Progenitor sequence of the assigned 28 sequences was generated by ancestral sequence reconstruction, and the generated sequence exhibited L-lysine oxidase activity; thus, we named the enzyme AncLLysO. AncLLysO has a fold typical of the flavin-dependent amine oxidase (FAO) superfamily —the Rossmann-core fold, which recognizes FAD, and a hot-dog-like fold, which is important for the recognition of substrates. Taken together, we assigned a novel FAD-dependent enzyme, called LLysO and bearing a main L-Lys α-oxidase and promiscuous monooxygenase activity, from the database. The main-chain amino group of L-Lys is deprotonated by an activated solvent water molecule, and the hydride on the main-chain carbon atom is transferred to FAD.

In this study, the crystal structure for the ligand-free form of AncLLysO (AncLLysO(LF)) was determined at a 2.4-Å resolution. The initial phase was determined using the iodide single anomalous dispersion (SAD) method. The active site structure of AncLLysO(LF) indicated that residues that would form interactions with the main-chain L-Lys are present including R76, G553, and W554. On the other hand, there is no space to bind L-Lys at the site as the side chain Y254 occupies the space, inferring that dynamic conformational changes of Y254 would be induced as the reaction progressed. In the ligand-free form, a cavity at the active site to recognize substrates is occupied by the side-chain Y254, which is the residue forming the plug loop; this occupation would bring about structural changes of the substrate recognition residues, such as E383 and Y516 and made it difficult to predict the recognition mechanism solely from the structure of the AncLLysO ligand-free form. Next, we attempted to represent structural changes of AncLLysO that are induced by the binding of substrates. Structural comparison between AncLLysO(LF)- (green) and the L-Lys-binding form of AncLLysO(K387A; magenta) are shown in Figure 5D, suggesting that dynamic structural changes could be confirmed at the following residues: 251 to 254, 383, and 516. From a structural comparison between the ligand-free form and the L-Lys- or L-Arg-binding form of AncLLysO, substrate binding appeared to induce a conformational change of a loop that is formed by residues 251 to 254 (251-GGYY-254); cis–trans transformation at G251 is remarkable in this change.

>MGNKNTPLNSGKHPDLKIEVAIIGAGTSGLYTAYRLVTDKKFKAHDVQIFDMNNKLGGRLESVIMPGMNFWGELGGMRYLTSQQIVTTLIEGYPLSEKDPNKRTPVLKDKMTPVPFPMGDPSKLLMYLRKERFKQNAWNEAQKKGEKLPTRYYLNENDLGFSSDQLFNKIIYDVLMADPWVAETYGSKIIKGSSVYDYSFKLTSRDWDDIKPKLVYNFPNSPYDQRKVNDIGFWNLIKDQVSQEGYEFLANAGGYYSNTINWNSAEAFPYMVGDFSAGTIYKTIEEGYDSIAYAVANSYMEHEGACIWSENKLLTFTKDHPLTNTHKYELTFLNLKTNTQWKVYANSIVLAMPRKSLELLDQNNFFFNINKNSVLNNNIRSVIMEPAFKILMGFEYPWWKELGIDSGHSITDLPMRQCYYFGTDPETNNSMLLGSYGDMETETFWKALSDDKVLFEVKAAKSASLRELHQLDDVQATKLMVGELMNQLRELHGDTVTIPEPYVTYFKDWTDEPFGAGYHAWKAGFSVENVMPYMRKPLTDEQIHICGEAYSDQQGWVEGAFCEAEKMLQEYFGLDRPYWLSPDYYLGWEHHHHHH[2x]>GSSHHHHHHSGDPASMNNHPEVKIKTILSLFLNINIDDFNMDANLADAYDMDXTELADLAKEIE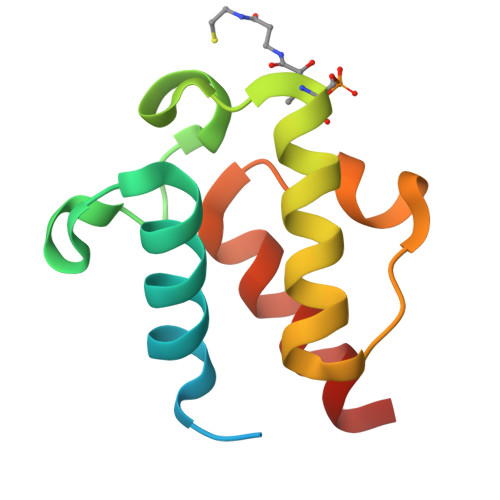KEFGISVTKSQFSHWETGRAVLDFVSSSLNDKN[2x]>GVHSFWDIAGPTARPVRLESLEDKRMAVDASIWIYQFLKAVRDQEGNAVKNSHITGFFRRICKLLYFGIRPVFVFDGGVPVLKRETIRQRKERRQGKRESAKSTARKLLANTTLSTSAERNVAENAFVEDELFEQQMKDKRDSDEVTMDMIKEVQELLSRFGIPYITAPMEAEAQCAELLQLNLVDGIITDDSDVFLFGGTKIYKNMFHEKNYVEFYDAESILKLLGLDRKNMIELAQLLGSDYTNGLKGMGPVSSIEVIAEFGNLKNFKDWYNNGQFDKRKQETENKFEKDLRKKLVNNEIILDDDFPSVMVYDAYMRPEVDHDTTPFVWGVPDLDMLRSFMKTQLGWPHEKSDEILIPLIRDV[2x]

Rad2/XPG belongs to the flap endonuclease family that encompasses various structure-specific nucleases involved in nucleic acid processing. The unique feature of Rad2/XPG is the recognition of DNA bubbles that comprise a stretch of unpaired bases flanked by double-stranded regions and correspond to the DNA in the NER pre-incision complex. We report four structures of the Rad2 catalytic core solved in four different space groups, three of which represent the productive substrate binding mode and reveal that the protein recognizes a single 5′ nucleotide of the single-stranded portion of the DNA and a 3′ phosphate group of the ss/dsDNA junction. The two critical regions for substrate binding are the H2TH module with a Rad2-specific α-helix 12b and the hydrophobic wedge that binds the first base pair of the double-stranded portion of the DNA.

Complex II was solved at 2.1 Å resolution and comprised two protein molecules, each interacting with one ss/dsDNA junction. The substrate used for crystallization contained 14 complementary bases with two-thymine single-stranded overhangs in all four DNA ends. However, in the crystal a single T-T mismatch formed, resulting in a 15-mer duplex with 1 nt overhangs in one end of the duplex and 2 nt overhangs in the other. For the non-cleaved (3′ flap) DNA strand, in one protein molecule of complex II and three protein molecules of complex III, we observed the electron density for the phosphate group of the ss/dsDNA junction. Several charged residues line a pocket located close to this phosphate: Arg60, Arg61 (both from the N region), His830 and Glu831 (from I region). In complex II, Arg60 and potentially Arg61 (through a water molecule) stabilize the phosphate at the junction. The productive complexes II–IV have the same overall architecture. The relative orientation of the protein molecules is similar between complexes II and III but differs in complex IV. All eight independently determined protein structures in complexes II–IV are essentially identical, with pairwise root-mean-square deviations (rmsds) between 0.5 and 0.8 Å over 273 to 285 C-α atoms. When all of the protein subunits from the productive complexes II–IV are compared, the DNA superimposes very well at the H2TH module, but its trajectory differs significantly in other regions, particularly around the hydrophobic wedge.5-(5-(4-(5-HYDRO-4-METHYL-2-OXAZOLYL)PHENOXY)PENTYL)-3-METHYL ISOXAZOLE | C19 H24 N2 O3 | 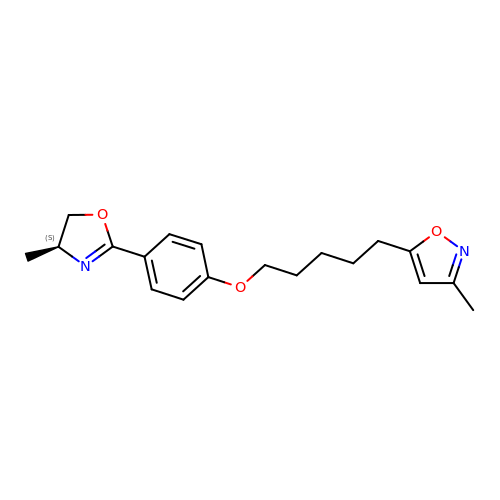UXIYKMARWUSIKU-HNNXBMFYSA-N> MGSSHHHHHSSGLVPRGSHMRYSLRQDIAVEPVIAGWYGWSYLLPPQTL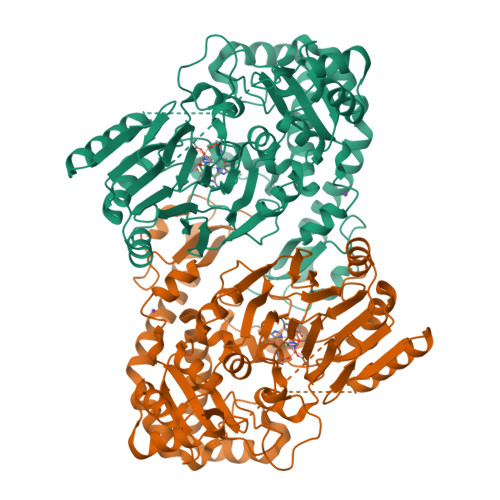ARFVHNRFNRIVESYLDDPQVHAAAVRQRRMHGGPWIHAHEHRDAIEAWYRETAPRRERLDELFEAVRRLEEDILPRHHGECLDPVYQELPAALAGRVEVFYGRDNRTADYRFVEPLMYASEYYDESWQQVRFRPVTEDAREFALTTPMLEYGPEQLLVNVPLNSPLLDAVFRGGLTGTELDDLAARFGLDGERAARFASYFEPTPAASEAPAPASSSEEDVLEYVGHACVFARHRGTTFLVDPVLSYSGYPGGAENRFTFADLPERIDHLLITHNHQDHMLFETLLRIRHRVGRVLVPKSTNASLVDPGLGGILRRLGFTDVVEVDDLETLSCGSAEVVALPFLGDHGDLRIRSKTGWLIRFGERSVLFAADSTNISPTMYTKVAEVIGPVDTVFIGMESIGAAASWIYGPLYGEPLDRRTDQSRRLNGSNFPQAREIVDALEPDEVYVYAMGLEPWMGVVMAVDYDESHPAIVDSDLLVRHVQDKGGTAERLHLRRTLRL> MCAGLPDQR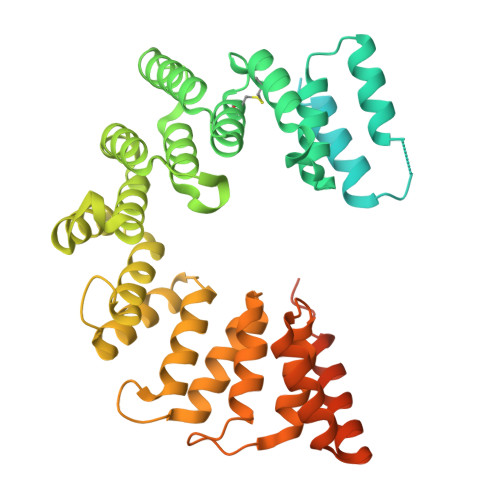LANEALKRGDTALAERNYKALADLGYSEAQVGLADIKVATRDPSQIKEAEATYRAAAATSPRAQARLGRLLVAKPDSTQAEREEAETLLKQAAKQGQSNTLIPLAMLYLSYPQSFPKVNAQQQIDQWRAAGNPEAGLAQVLLYRTQGTYDQHLGEVEKICKAALNTTDICYVELATVYQKRGQADQQAALLGQLKSAYARGAVPATRVDSVARVLADRSLGQTDEKTAKELLEQVAPANPASWVSLAQLVYDFPELGDTDQLMAYIDKGREAEQPRAELLLGRLYYEGKTLPADAQKAEQHLQAAAEAGEISAHYYLGQLYRRGYLGNVEPQKAVDHLLAAARGGQNSADYALAQLFSEGHGIRPQPGNAWVFAQLSQANPTPQSAELLQQLDQQLTPDQRNQAQQLLDQEKRARGSLAQGANSTLALEALQDDEKEVDGEDSLLEHHHHHH>MDNGELISIIVPVYNVEKYLKRCLDSLLRQTYKNFEIILINDGSTDNSSIICEEYAKIDNRIQILHQTNAGPSAARNAGITYASGKYITFVDSDDFVEEFYLEHLYRALVDNGSDISVCNFNSFNEDRQSFLFSITKEKYFCKNYTIAEWMDLESSANNNLFLTFTFSPTKLFKAELFEGIRFPLGRLREDDATIYRLYLKASQITFINEGSYYYSQRSEGLSRTRMLDDISSMISNAEERIALLASMGYDLTEQIKSYKGRLKKCCEDALRNGQIELYQQCCNKLDLIENYPKE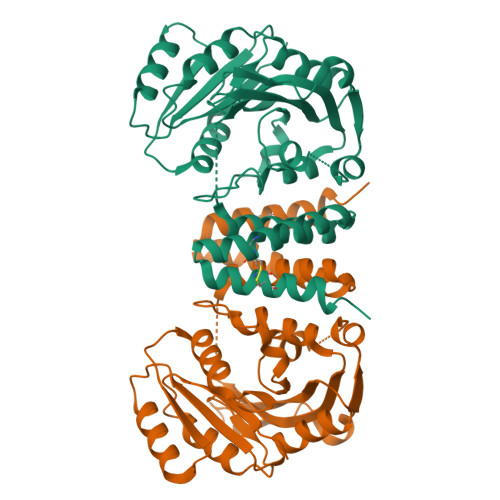K[2x]> GPLGSGRPQSERNYLWREENAEQQA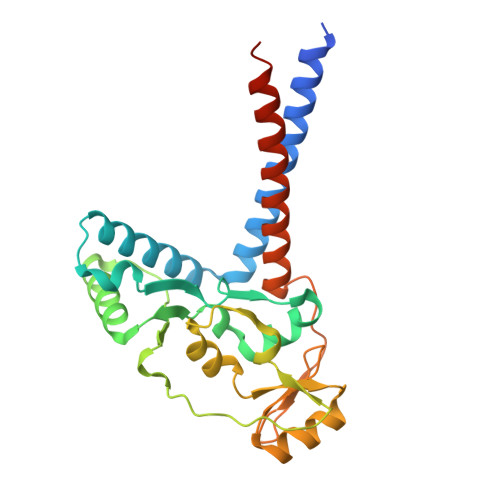LAAKREDLEKKQQLLRAATGKAILNGIDSINKVLDHFRRKGINQHVQNGYHGIVMNNFECEPAFYTCVEVTAGNRLFYHIVDSDEVSTKILMEFNKMNLPGEVTFLPLNKLDVRDTAYPETNDAIPMISKLRYNPRFDKAFKHVFGKTLICRSMEVSTQLARAFTMDCITLEGDQVSHRGALTGGYYDTRKSRLELQKDVRKAEEELGELEAKLNENLRRNIERINNEIDQ>QAQITGRPEWIWLALGTALMGLGTLYFLVKGMGVSDPDAKKFYAITTLVPAIAFTAYLSMLLGYGLTMVPFGGEQNPIYWARYADWLFTTPLLLLDLALLVDADQGTILALVGADGIMIGTGLVGALTKVYSYRFVWWAISTAAMLYILYVLFFGFTSKAESMRPEVASTFKVLRNVTVVLWSAYPVVWLIGSEGAGIVPLNIETLLFMVLDVSAKVGFGLILLRSRAIFGEAEAPEPSA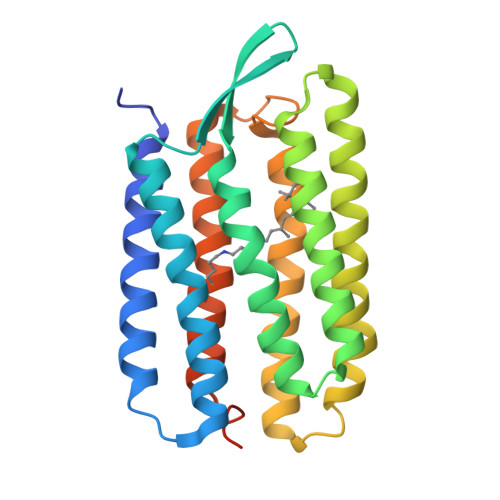GDGAAATSD[2x]> AFYKREMFDPAEKYKMDHRRRGIALIFNHERFFWHLTLPERRGTCADRDNLTRRFSDLGFEVKCFNDLKAEELLLKIHEVSTVSHADADCFVCVFLSHGEGNHIYAY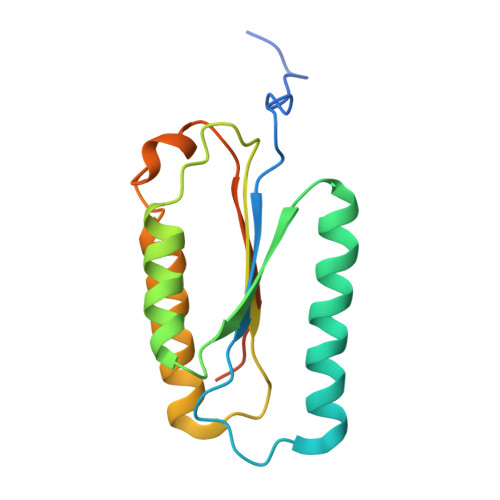DAKIEIQTLTGLFKGDKCHSLVGKPKIFIIQACRGNQHDVPVIPLDVVD>MMSDQENENEHAKAFLGLAKCEEEVDAIEREVELYRLNKMKPVYEKRDAYIDEIAEFWKIVLSQHVSFANYIRASDFKYIDTIDKIKVEWLALESEMYDTRDFSITFHFHGIEGDFKEQQVTKVFQIKKGKDDQEDGILTSEPVPIEWPQSYDSINPDLIKDKRSPEGKKKYRQGMKTIFGWFRWTGLKPGKEFPHGDSLASLFSEEIYPFCVKYYAEAQRDLEDEEGESGLSADGDSEDDDGSLGEVDLPLSDEEPSSKKRKV[4x]

Vacuolar Protein Sorting 75 (Vps75) is a histone chaperone belonging to the Nucleosome Assembly Protein (NAP-1) family. However, Vps75 is best known for its ability to stimulate the histone H3 acetyl transferase activity of Regulator of Ty1 Transposition 109 (Rtt109) in Saccharomyces cerevisiae. All crystal structures published to date show Nap1 (5,6) and Vps75 (7–9) to be homo-dimeric proteins adopting characteristic ‘headphone’ folds, in which a long N-terminal helix self-associates in an antiparallel manner to form the dimerization interface which is capped at either end by a globular domain. In addition to the headphone fold, both Nap1 and Vps75 contain C-terminal acidic domains dispensable for histone binding.

While attempting to crystallize Vps75 in complex with histones H3–H4, we inadvertently crystallized Vps75 with four Vps75 monomers in the asymmetric unit. Upon repetition of the asymmetric unit, two distinct tetrameric assemblies of Vps75 are clearly observed in the crystal lattice. One tetramer is made up of two dimers of Vps75, each composed of a copy of chains A and B, which together form an asymmetric ring-like tetramer. The second, symmetrical ring-like tetramer, is composed of a dimer of chain C and a dimer of chain D. Both tetramers are related structures, with the latter most closely resembling the conformation previously observed in solution. In the symmetrical tetramer, the antiparallel dimerization helices of one dimer form a saltire-like cross with those of the opposing dimer (top middle). A ∼30° dislocation in the register of the two dimers allows the symmetrical tetramer to transition into the asymmetrical tetramer (bottom middle) and vice versa. In the symmetrical tetramer the ring-like cavity is open at both sides (top left). However, the transition to the asymmetrical tetramer is also accompanied by a closure of one side of the cavity as the globular domain of one dimer occupies the cavity of the opposing dimer and vice versa (bottom left). Amino-acid conservation analysis shows that residues mapping to the asymmetric and symmetric tetramerization interfaces of Vps75 are well conserved. Thus, in the tetrameric conformation, dimers of Vps75 have a relatively large acidic concave groove between the globular domains of each Vps75 monomer as a result of a straightening of the antiparallel dimerization helices.>MTRILAPIPSPPKHPQYGHLHYLAGDAPVLNFFQLARQIPEGLFQLDIQGRTLIQAYDPNLVAELTDERRFQKRVHPAYTNIRNLGGDGLFTSDSFEPNWGKAHRILLPAFSQRAMKGYFGQMLEVAQALVGKWERTQGQDVRVADDMTRLTLDTISLSGFDYRFRSFDKDELHPFLQALARAMHHTMTMFSRPPVLTPEMEEADRAYWADIASMNELVDEVIRERRGHGGGGGDLLGLMLNATDPETGERLSDENIRYQVMTFLIAGHETTSGLLAFTLYLLLRHPHVLAQAYAEVDRLLPGDAVPTYDTVMRLDVIPRILDEALRFWSTIPNYAVTALQDEVIGGKYEIRKGQQLALLIPALHRHPAAWTNPDEFDIDRW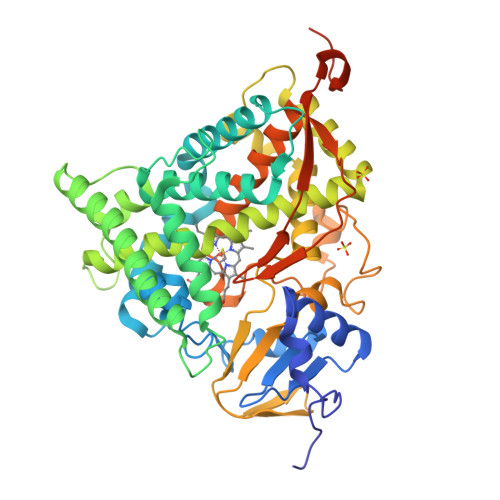TSENRRTHHPAAYKPFGNGMRACIGRQFALTEAKLALLLILQKFALSDPYDYHLKVKQSLTIKPEDFALRVRERRPHERFSVPVPVVEEPQQDLSRVSVAGTGVELTVAYG[4x]>[4x]MMMKFINIGYGNMVSAARIITIVSPDSAPIKRIIQDAREKGKLVDATHGRRTRAVIITDSDHVILSSVQPETVANRLYGSDDFSEEG

Bacillus subtilis can form structurally complex biofilms on solid or liquid surfaces, which requires expression of genes for matrix production. The transcription of these genes is activated by regulatory protein RemA, which binds to poorly conserved, repetitive DNA regions but lacks obvious DNA-binding motifs or domains. Here, we present the structure of the RemA homologue from Geobacillus thermodenitrificans, showing a unique octameric ring with the potential to form a 16-meric superstructure. These results, together with further biochemical and in vivo characterization of B. subtilis RemA, suggests that the protein can wrap DNA around its ring-like structure through a LytTR-related domain.

The structure of (Gt)RemA was determined at 2.3 Å resolution by selenium single-wavelength anomalous diffraction (Se-SAD), because no appropriate search model could be identified. Amino acids 2–83 of (Gt)RemA could be unambiguously assigned into the electron density map. Analysis of the crystallographic asymmetric unit showed that four RemA monomers arranged into a tetramer reminiscent of a semicircle. Following the crystallographic 2-fold rotation axis, the other half of the semicircle is found in the neighboring asymmetric unit across the crystallographic two-fold axis. Thus, our structural analysis, consistent with our biochemical analysis, shows that 8 monomers of RemA form a donut-shaped 8-mer with outer dimensions of approximately 71 and 35 Å and a central hole of approximately 20 Å in diameter. Central for the interaction of two monomers within the ring is the β-sheet augmentation of β2 of one monomer with β3 of the adjacent monomer. Closer inspection of our RemA structure with the aim to identify its putative DNA-binding motif(s) or domain(s) revealed an extended, positively charged surface on the outside of the 8-mer. Moreover, this surface coordinates three sulfate ions (i.e., S1 to S3) originating from the crystallization buffer. These sulfate ions are primarily coordinated by the positively charged arginines 50, 51, and 53. Two (RemA)8 rings are always stacked ‘back-to-back’ to form 16-mers.(3R)-1-pyrrolo[1,2-a]quinoxalin-4-ylpiperidine-3-carboxylic 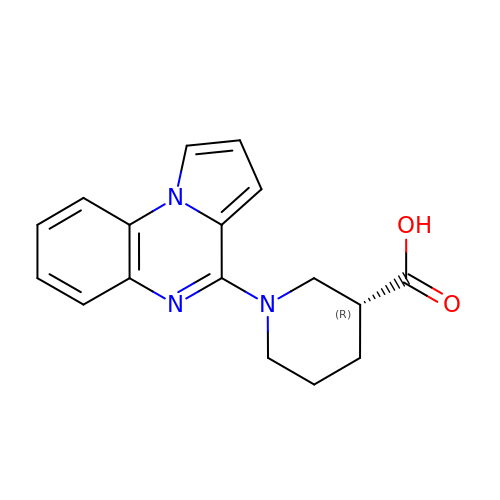acid | C17 H17 N3 O2 | IJWLQMUBOJDFNL-GFCCVEGCSA-N> MVDAVVTVFLEKTLNILEEKGRTVSDYRKQLEDLQSELKYMQSFLKDAERQKRTNETLRTLVADLRELVYEAEDILVDCQLADGDDGNEQRSSNAWLSRLHPARVPLQYKKSKRLQEINERITKIKSQVEPYFEFITPSNVGRD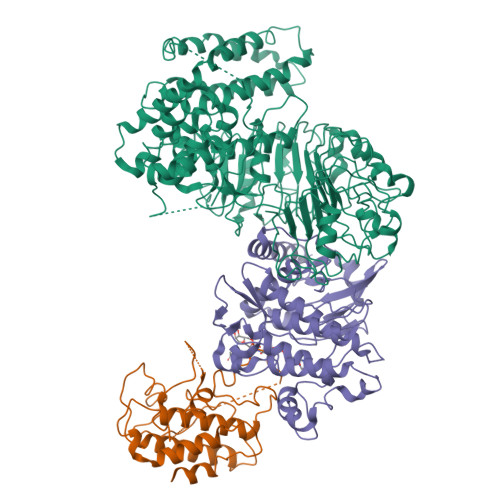NGTDRWSSPVYDHTQVVGLEGDKRKIKEWLFRSNDSQLLIMAFVGMGGLGKTTIAQEVFNDKEIEHRFERRIWVSVSQTFTEEQIMRSILRNLGDASVGDDIGTLLRKIQQYLLGKRYLIVMDDVWDKNLSWWDKIYQGLPRGQGGSVIVTTRSESVAKRVQARDDKTHRPELLSPDNSWLLFCNVAFAANDGTCERPELEDVGKEIVTKCKGLPLTIKAVGGLLLCKDHVYHEWRRIAEHFQDELRGNTSETDNVMSSLQLSYDELPSHLKSCILTLSLYPEDCVIPKQQLVHGWIGEGFVMWRNGRSATESGEDCFSGLTNRCLIEVVDKTYSGTIITCKIHDMVRDLVIDIAKKDSFSNPEGLNCRHLGISGNFDEKQIKVNHKLRGVVSTTKTGEVNKLNSDLAKKFTDCKYLRVLDISKSIFDAPLSEILDEIASLQHLACLSLSNTHPLIQFPRSMEDLHNLQILDASYCQNLKQLQPCIVLFKKLLVLDMTNCGSLECFPKGIGSLVKLEVLLGFKPARSNNGCKLSEVKNLTNLRKLGLSLTRGDQIEEEELDSLINLSKLMSISINCYDSYGDDLITKIDALTPPHQLHELSLQFYPGKSSPSWLSPHKLPMLRYMSICSGNLVKMQEPFWGNENTHWRIEGLMLSSLSDLDMDWEVLQQSMPYLRTVTANWCPELESFAIEDVGFRGGVWMKTPLHRT;> MKKQYLKSGSGTRKEKDKAKRWFLDNGSIFLRELVADCNGKSIPIRSFSPEQILKATNNFDSSCFVSQDVYYKWYRGEIEDRSYMIKRFSEDEITGKRHRVKEVYNDIVLSARMSNHSNFLQLLGCCLEFPFPVLVFEFAEHGAMNQRGGVIVNGEESLLPWSVRLKIGKEIANAVTYLHTAFPKIIIHRDVKPMHVFLDKNWTAKLSDLSFSISLPEGKSRIEAEWVLGTFGYIDPLYHKTCFVTEYTDVYSFGICLLVIITGKPAIMTISDGDLQGILSLVRELCENGKLDEVIDPRLMKDITSGQRLQVEACVVLALRCCKERDEDRPKMIQVAKELKQIEASLKNSS;> MGNCLDSSAKVDNSNHSPHANSASSGSKVSSKTSRSTGPSGLSTTSYSTDSSFGPLPTLRTEGEILSSPNLKAFTFNELKNATKNFRQDNLLGEGGFGCVFKGWIDQTSLTASRPGSGIVVAVKQLKPEGFQGHKEWLTEVNYLGQLSHPNLVLLVGYCAEGENRLLVYEFMPKGSLENHLFRRGAQPLTWAIRMKVAVGAAKGLTFLHEAKSQVIYRDFKAANILLDADFNAKLSDFGLAKAGPTGDNTHVSTKVIGTHGYAAPEYVATGRLTAKSDVYSFGVVLLELISGRRAMDNSNGGNEYSLVDWATPYLGDKRKLFRIMDTKLGGQYPQKGAFTAANLALQCLNPDAKLRPKMSEVLVTLEQLESVAKPGTKHTQMESPRFHHSSVMQKSPVRYSHDRPLLHMTPGASPLPSYTQSPRVR> MVGNREEKILNREIGFAIGMPVCEFDMVKDPEVQDFRRNILNVCKEAVDLRDLNSPHSRAMYVYPPNVESSPELPKHIYNKLDKGQIIVVIWVIVSPNNDKQKYTLKINHDCVPEQVIAEAIRKKTRSMLLSSEQLKLCVLEYQGKYILKVCGCDEYFLEKYPLSQYKYIRSCIMLGRMPNLMLMAKESLYSQLPMDCFTMPSYSRRISTATPYMNGETSTKSLWVINSALRIKILCATYVNVNIRDIDKIYVRTGIYHGGEPLCDNVNTQRVPCSNPRWNEWLNYDIYIPDLPRAARLCLSICSVKGRKGAKEEHCPLAWGNINLFDYTDTLVSGKMALNLWPVPHGLEDLLNPIGVTGSNPNKETPCLELEFDWFSSVVKFPDMSVIEEHANWSVSREAGFSYSHAGLSNRLARDNELRENDKEQLKAISTRDPLSEITEQEKDFLWSHRHYCVTIPEILPKLLLSVKWNSRDEVAQMYCLVKDWPPIKPEQAMELLDCNYPDPMVRGFAVRCLEKYLTDDKLSQYLIQLVQVLKYEQYLDNLLVRFLLKKALTNQRIGHFFFWHLKSEMHNKTVSQRFGLLLESYCRACGMYLKHLNRQVEAMEKLINLTDILKQEKKDETQKVQMKFLVEQMRRPDFMDALQGFLSPLNPAHQLGNLRLEECRIMSSAKRPLWLNWENPDIMSELLFQNNEIIFKNGDDLRQDMLTLQIIRIMENIWQNQGLDLRMLPYGCLSIGDCVGLIEVVRNSHTIMQIQCKGGLKGALQFNSHTLHQWLKDKNKGEIYDAAIDLFTRSCAGYCVATFILGIGDRHNSNIMVKDDGQLFHIDFGHFLDHKKKKFGYKRERVPFVLTQDFLIVISKGAQECTKTR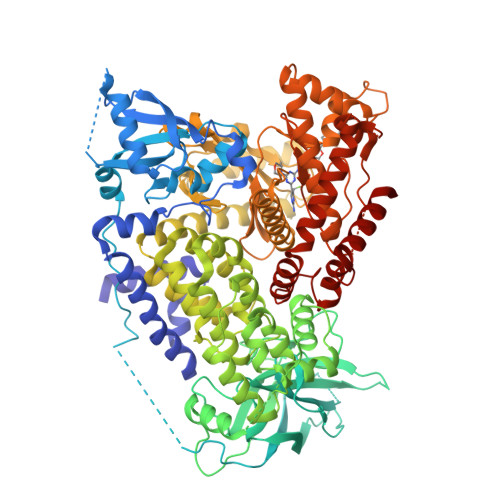EFERFQEMCYKAYLAIRQHANLFINLFSMMLGSGMPELQSFDDIAYIRKTLALDKTEQEALEYFMKQMNDAHH>[2x]QSLVADVGDDHHAW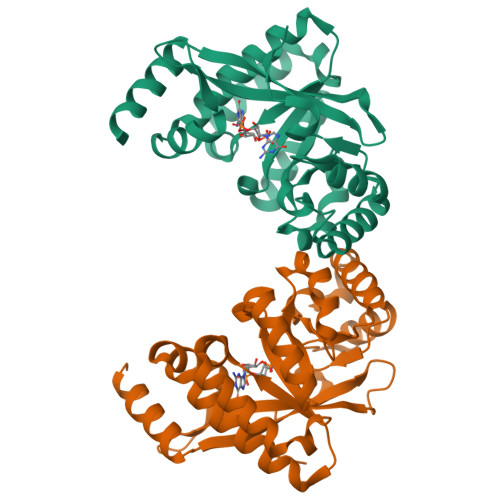HRLLDQALNQRRFELFFQPVVAAQDTQLVLHYKVLSRLLDEQGQTIPAGRFLPWLERFGWTARLDRLMLERVLEQMAGHEESLALNLSSATLADPQALNKVFEILRAHSNLGARLTLEIGEEQLPEQAVLEQLTRRLRELGFSLSLQRFGGRFSMIGNLARLGLAYLKIDGSYIRAIDQESDKRLFIEAIQRAAHSIDLPLIAERVETEGELSVIREMGLYGVQGQLFGEPKPWG>SGMGGIT[2x]

Although other intermediate filament proteins have been demonstrated to form amyloids, KRT8 specifically has not previously been characterized as an amyloid-forming protein. This protein, like other alpha-keratin proteins, contains a central coiled-coil domain that is flanked by an amino-terminal head domain and a carboxy-terminal tail domain, which are both low complexity in sequence composition. KRT8 is known to aggregate pathologically, primarily in the form of MDBs in liver disease. Atomic structures of KRT8 LARKS reveal that pathogenic mutations convert the non-pleated wild-type protein into a pleated conformation, shedding light on the molecular mechanisms underlying aggregation-promoting mutations in low-complexity proteins.

To assess the structural impacts of the disease-associated mutations, we determined the atomic structures of several LARKS from KRT8 for both the wild-type and mutant sequences. Segment crystal structures of KRT858–64 (wild type: SGMGGIT; G62C: SGMGCIT) for the wild-type protein and KRT8-G62C were determined. The wild-type fibril contains an anti-parallel beta-sheet, with PEG and ethanol molecules bound along the fibril axis. The central glycine residues (Gly61 and Gly62) adopt a nearly linear beta-strand conformation. Alignment of the beta-strands from both structures highlights that the G62C mutation results in the non-pleated Gly62 converting to a pleated conformation as Cys62 (shown in inset). e, Comparison of the KRT852-58-G55A GGYAGAS segment with a structure from hnRNPA1 whose sequences closely match the corresponding KRT8 wild-type (hnRNPA1: GGGYGGS versus KRT8: GGYGGAS) shows a similar trend in transitioning from an extended beta-sheet in the wild type to a pleated conformation in the mutant. An overlay of both wild-type–mutant structure pairs highlights that mutations from wild-type glycines facilitate a transition in the backbone from a non-ideal, highly extended conformation to a pleated one. Suggesting an effect of alcohol on KRT8 aggregation, two of three of our crystal structures of KRT8 segments showed the peptides in complex with either ethanol or isopropanol, each with distinct binding sites. The wild-type SGMGGIT structure (a) shows two ethanol molecules (gray) per asymmetric unit coordinated to the N terminus of the peptide, while mutant SGMGCIT (b) displays isopropanol binding alongside the middle of the peptide along the fibril axis, occupying the space between the beta-sheets (in gray) in the steric zipper. Both structures illustrate that alcohols can directly associate with KRT8 amyloid fibrils.> MKRSDKHGKNRTGAYIAGAVILIAAAGGGYFYYQHYQETQAVEAGEKTVEQFVQALNKGDYNKAAEMTSKKAANKSALSEKEILDKYQNIYGAADVKGLQISNLKVDKKDDSTYSFSYKAKMNTSLGELKDLSYKGTLDRNDGQTTINWQPNLVFPEMEGNDKVSLTTQEAARGNIIDRNGEPLATTGKLKQLGVVPSKLGDGGEKTANIKAIASSFDLTEDAINQAISQSWVQPDYFVPLKIIDGATPELPAGATIQEVDGRYYPLGEAAAQLIGYVGDITAEDIDKNPELSSNGKIGRSGLEMAFDKDLRGTTGGKLSITDADGVEKKVLIEHEVQNGKDIKLTIDAKAQKTAFDSLGGKAGSTVATTPKTGDLLALASSPSYD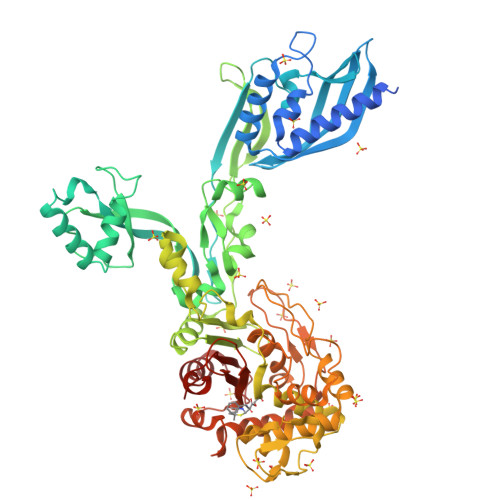PNKMTNGISQEDYKAYEENPEQPFISRFATGYAPGSTFKMITAAIGLDNGTIDPNEVLTINGLKWQKDSSWGSYQVTRVSDVSQVDLKTALIYSDNIYTAQETLKMGEKKFRTGLDKFIFGEDLDLPISMNPAQISNEDSFNSDILLADTGYGQGELLINPIQQAAMYSVFANNGTLVYPKLIADKETKDKKNVIGETAVQTIVPDLREVVQDVNGTAHSLSALGIPLAAKTGTAEIKEKQDVKGKENSFLFAFNPDNQGYMMVSMLENKEDDDSATKRASELLQYLNQNYQ> METELSPNLPLPIYYTYPNSLTL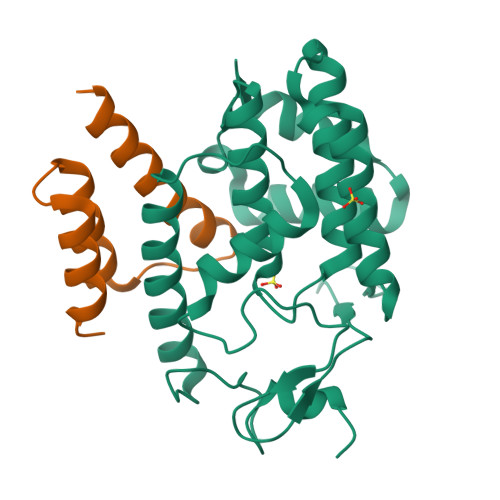KNKYGIIDHKEFTDKCAHDSAKATINLHQEALPKEFNSSYLKYLHKCLFENTFEWAGCTRDIPFPFKDGTVAVMPEMMRSNWKTDQPIIFAIGNKVQDGLKNIDRILVEKNNLQNLPRQEFIHHLAEIFASLNYTHPFREGNGRTQRIFCEKLAQAANYNLDFSIVTKERMSEVSIAAAQDGNLEPMKKLFDDISHHHHHH;> VKKTTDHSTSLTSEELQKRREAVDAAISTHAIEGITLHSKTLEILEGYAKGEYSLEEFNTLMDNATL> GLPVLNTPGSNQYLTSDNYQSPCAIPEFDVTPPIDIPGEVKNMMELAEIDTMIPLNLENTKR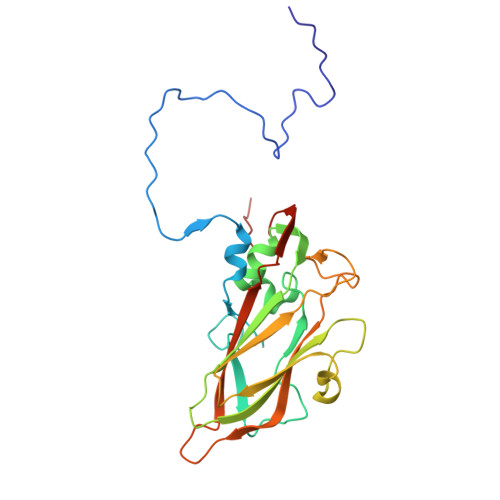NTMDMYRVTLSDSADLSQPILCFSLSPASDPRLSHTMLGEVLNYYTHWAGSLKFTFLFCGSMMATGKILVAYAPPGAQPPTSRKEAMLGTHVIWDLGLQSSCTMVVPWISNVTYRQTTQDSFTEGGYISMFYQTRIVVPLSTPKSMSMLGFVSACNDFSVRLLRDTTHISQSALPQ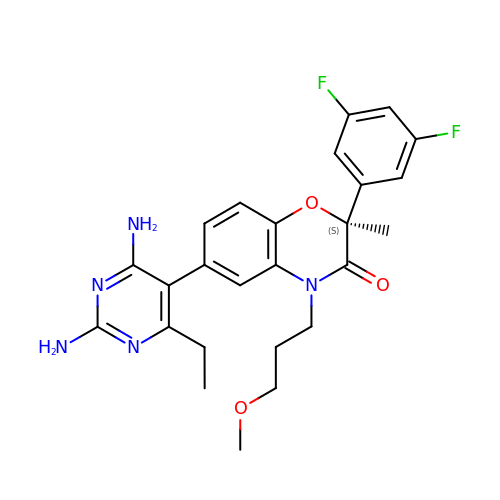(2S)-6-(2,4-DIAMINO-6-ETHYLPYRIMIDIN-5-YL)-2-(3,5-DIFLUOROPHENYL)-4-(3-METHOXYPROPYL)-2-METHYL-2H-1,4-BENZOXAZIN-3(4H)-ONE | C25 H27 F2 N5 O3 | UAXNNGUDPWZOKX-VWLOTQADSA-N>APRQHLLSLTRRAQKHRLRELKIQVKEFADKEEGGDVKAVCLTLFLLALRARNEHRQADELEAIMQGRGSGLQPAVCLAIRVNTFLSCSQYHKMYRTVKAITGRQIFQPLHALRNAEKVLLPGYHPFEWQPPLKNVSSRTDVGIIDGLSGLASSVDEYPVDTIAKRFRYDSALVSALMDMEEDILEGMRSQDLDDYLNGPFTVVVKESCDGMGDVSEKHGSGPAVPEKAVRFSFTVMRITIEHGSQNVKVFEEPKPNSELCCKPLCLMLADESDHETLTAILSPLIAEREAMKSSELTLEMGGIPRTFKFIFRGTGYDEKLVREVEGLEASGSVYICTLCDTTRLEASQNLVFHSITRSHAENLQRYEVWRSNPYHESVEELRDRVKGVSAKPFIETVPSIDALHCDIGNAAEFYKIFQLEIGEVYKHPNASKEERKRWQATLDKHLRKRMNLKPIMRMNGNFARKLMTQETVDAVCELIPSEERHEALRELMDLYLKMKPVWRSSCPAKECPESLCQYSFNSQRFAELLSTKFKYRYEGKITNYFHKTLAHVPEIIERDGSIGAWASEGNE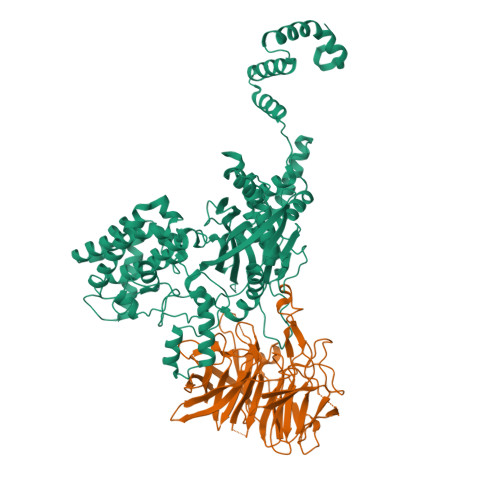SGNKLFRRFRKMNARQSKCYEMEDVLKHHWLYTSKYLQKFMNAHNA[2x];>[2x]SLQMVTVGHNIALIQPGFSLMNFDGQVFFFGQKGWPKRSCPTGVFHFDIKQNHLKLKPAIFSKDSCYLPPLRYPATCSYKGSIDSDKHQYIIHGGKTPNNELSDKIYIMSVACKNNKKVTFRCTEKDLVGDVPEPRYGHSIDVVYSRGKSMGVLFGGRSYMPSTQRTTEKWNSVADCLPHVFLIDFEFGCATSYILPELQDGLSFHVSIARNDTVYILGGHSLASNIRPANLYRIRVDLPLGTPAVNCTVLPGGISVSSAILTQTNNDEFVIVGGYQLENQKRMVCSLVSLGDNTIEISEMETPDWTSDIKHSKIWFGSNMGNGTIFLGIPGDNKQAMSEAFYFYTLRC> ETGSAQQLNEDLRLHLLLNTSVTCNDGSPAGYYLKESRGSRRWLLFLEGGWYCFNRENCDSRYDTMRRLMSSRDWPRTRTGTGILSSQPEENPYWWNANMVFIPYCSSDVWSGASSKSEKNEYAFMGALIIQEVVRELLGRGLSGAKVLLLAGSAAGGTGVLLNVDRVAEQLEKLGYPAIQVRGLADSGWFLDNKQYRHTDCVDTITCAPTEAIRRGIRYWNGVVPERCRRQFQEGEEWNCFFGYKVYPTLRSPVFVVQWLFDEAQLTVDNVHLTGQPVQEGLRLYIQNLGRELRHTLKDVPASFAPACLSHEIIIRSHWTDVQVKGTSLPRALHCW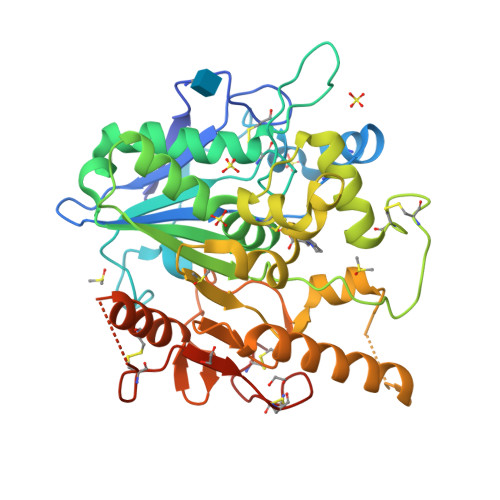DRSLHDSHKASKTPLKGCPVHLVDSCPWPHCNPSCPTGTKHHHHHH>[2x]ALYEDPPDQKTSPSGKPATLKICSWNVDGLRAWIKKKGLDWVKEEAPDILCLQETKCSENKLPAELQELPGLSHQYWSAPSDKEGYSGVGLLSRQAP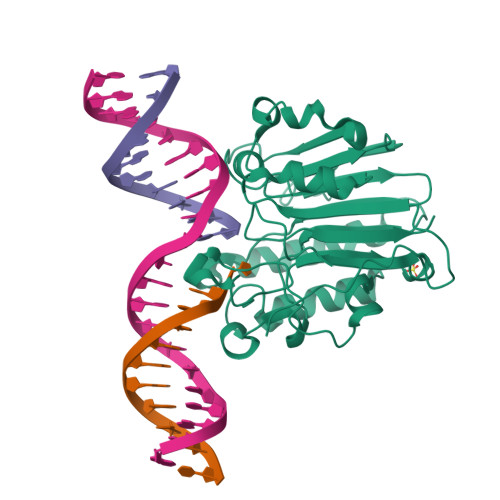LKVSYGIGDEEHDQEGRVIVAEFDSFVLVTAYVPDAGRGLVRLEYRQRWDEAFRKFLKGLASRKPLVLCGDLNVAHEEIDLRNPKGNKKNAGFTPQERQGFGELLQAVPLADSFRHLYPNTPYAYTFWTYMMNARSKNVGWRLDYFLLSHSLLPALCDSKIRSKALGSDHCPITLYLAL> MDNLTKVREYLKSYSRLDQAVGEIDEIEAQRAEKSNYELFQEDGVE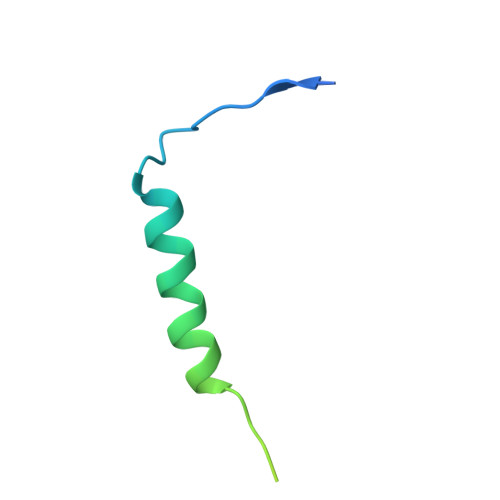EHTKPSYFQAADDSLEHHHHHH CDK16 is a newly recognised member of the CDK protein kinase family that is activated upon binding to the membrane-associated protein cyclin Y (CCNY) or its homologue cyclin Y-like 1 (CCNYL1). The crystal structures of monomeric CDK16 represent the first structures from the PCTAIRE family of CDK kinases. The kinase domain exhibits the classical bilobal architecture intermixed with short insertions that help to define the CDK family fold. The predominantly α-helical C-lobe contains the CDK/MAPK insert, which packs against the αDE and αG helices, as well as a PCTAIRE family specific C-terminal extension that stretches behind the αI helix before folding back to terminate beside the αD helix.

Viable crystals were first obtained for a complex containing the type I inhibitor indirubin E804. The structure of this complex was solved using CDK5 as a phasing model and refined at a resolution of 2.4 Å with one CDK16 monomer in the asymmetric unit. The complex with indirubin E804 displays some disorder in the kinase N-lobe, consistent with its requirement for a cyclin partner. However, in the indirubin E804 complex, the αC is reduced to a single helical turn and the preceding PCTAIRE motif instead adopts a loosely extended conformation that is stabilised by crystal packing. In particular, the partial unfolding of the αC helix in the indirubin E804 co-structure suggests that the isolated CDK16 kinase domain may be relatively unstable in the absence of a cyclin partner. The indirubin E804 scaffold is largely planar and binds to the kinase hinge region of CDK16 using three hydrogen bonds, including two from the indole-2-one moiety and one from the indole moiety. These groups also present a significant hydrophobic surface for van der Waals interactions with the ATP pocket residues Leu171, Val179, Ala192, Val224, Phe240, Leu293 and Ala303. The hydroxybutyloxime moiety extends across the expected ribose- and phosphate-binding sites of the ATP pocket. Here, the flipped-out conformation of Phe305 in the activation segment establishes a cage-like structure around the inhibitor. The binding therefore features an induced fit that maximises the kinase–inhibitor interaction.

> METYIKLDKLGEGTYATVYKGKSKLTDNLVALKEIRLEHEEGAPCTAIREVSLLKDLKHANIVTLHDIIHTEKSLTLVFEYLDKDLKQYLDDCGNIINMHNVKLFLFQLLRGLAYCHRQKVLHRDLKPQNLLINERGELKLADFGLARAKSIPTKTYDNEVVTLWYRPPDILLGSTDYSTQIDMWGVGCIFYEMATGRPLFPGSTVEEQLHFIFRILGTPTEETWPGILSNEEFKTYNYPKYRAEALLSHAPRLDSDGADLLTKLLQFEGRNRISAEDAMKHPFFLSLGERIHKLPDTTSIFALKEIQLQKEASLRSAHHHHHH1-(cyclohexylamino)-7-(1-methyl-1H-pyrazol-4-yl)-5H-pyrido[4,3-b]indole-4-carboxamide | C22 H24 N6 O | 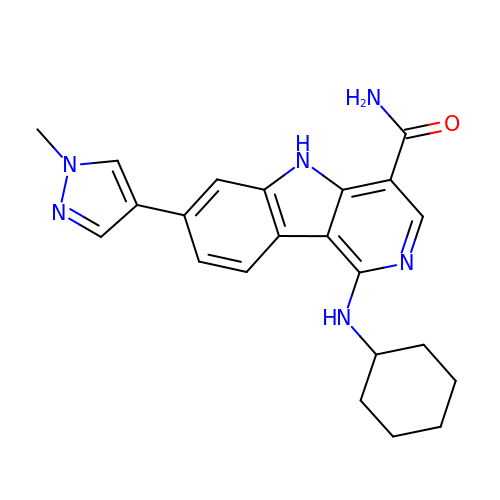NSYNFVRSQTTZAL-UHFFFAOYSA-N>[15x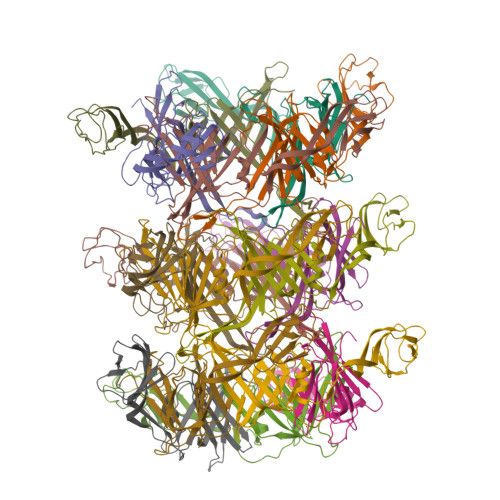]MKTVIQDTADVYFKRKSDGKLVFTAEAQTASFSQAISEEKLRGGIGNKPLYILKSEKEINLTVKNAFFDLEWLAMTQGETIQEETKVKVFDREHGLIVDDTNKVTLKGKPVSDVTFYNKKGLTYKIAVSTDGTYTIPTAFAAAKDKLTAVYQIEKVGRRLAIKASKFSERYEVEYRTIAYNPDTEEVYSDIYIQFPNVSPSGEFEMSLENGNALAPEIKFEALADTDTDEMAVVIEASRDENTAAPVEDTTGSTQSSDLGGTTEHHHHHH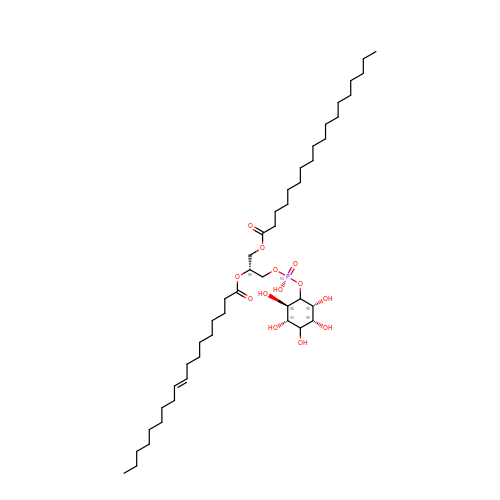(1R)-2-{[(S)-hydroxy{[(1S,2R,3R,4S,5S,6R)-2,3,4,5,6-pentahydroxycyclohexyl]oxy}phosphoryl]oxy}-1-[(octadecanoyloxy)methyl]ethyl (9Z)-octadec-9-enoate | C45 H85 O13 P | YOBFISPJJWPPTK-BAAZTTAESA-N3-{[(4-chlorophenyl)acetyl]amino}pyridine-4-carboxylic acid 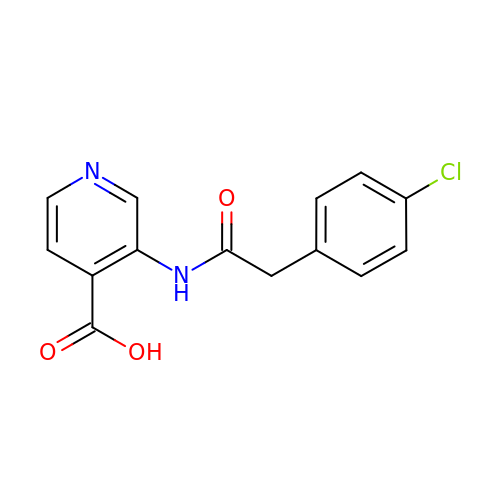| C14 H11 Cl N2 O3 | BGMIWCIVXVXHDU-UHFFFAOYSA-N>[2x]MQSYSRRWFLGAGATTLISAAGLTACGSGSGSGGSGGTITAMVYGDDAVKVQDKAASRFNASAEAKKANAKVKMERIPASDYPAKLRTAMGSPNAPDIFFNWGGGSIKAYKEAGQLVDLTDVIKSDEVLSTGFLPSVVAAGSLDGHEYGIPMRGMQPVLLFYNKSVFAEHKLTPPTTWDQLLDNVAKLKKAGVT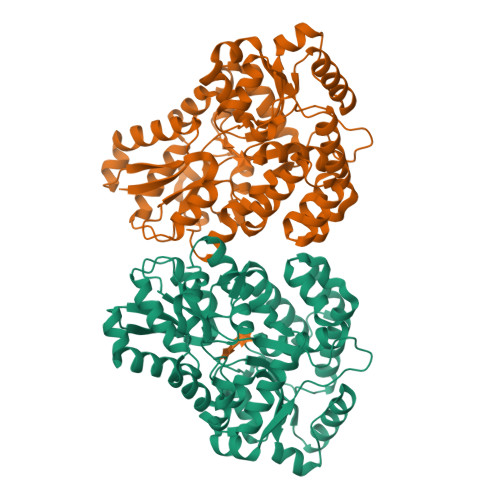PFALGGVEIWPELMWLEYLVDRIGGPQVFDKIRNGDASGWGDPAVLKAAQTVKQLVDEGAFGKGFSSVSYNNGGAPALLAKGKAGMHLMGSWEYSTQLGKFPDFAKKDLGWCAFPSFEGGAGDIRNVVGNPCNYWSVNARTGNKDGAIAFLRDCASEAYTKDLIDNGDVPTTTIAENMLDSSPNPEFAKFQYQLVQKAPNFTLSWDQAVDPDWQQPMLTEINKLFVGKSSPEQFVSALKGLK>MRPDLSRVPGVLGEIARKRASEVAPYPLPEPPSVPSFKEALLRPGLSVIAEVKRQSPSEGLIREVDPVE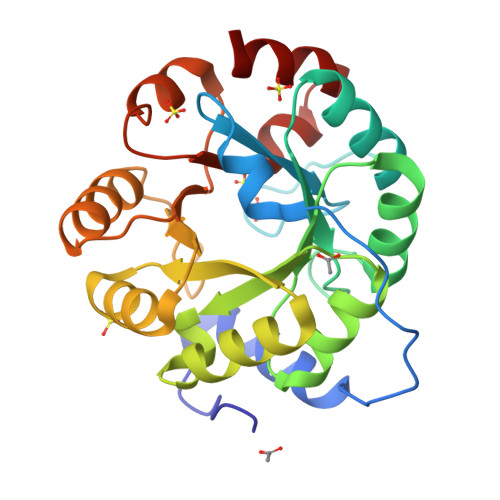AALAYARGGARAVSVLTEPHRFGGSLLDLKRVREAVDLPLLRKDFVVDPFMLEEARAFGASAALLIVALLGELTGAYLEEARRLGLEALVEVHTERELEIALEAGAEVLGINNRDLATLHINLETAPRLGRLARKRGFGGVLVAESGYSRKEELKALEGLFDAVLIGTSLMRAPDLEAALRELVG[2x]>XNLAALRSELQALRREGFSPERLAALESRLQALERRLAALRSRLQALRGX[4x];>XGLCALRSELQALRREGFSPEELAALESELQALERELAALRSELQALRGX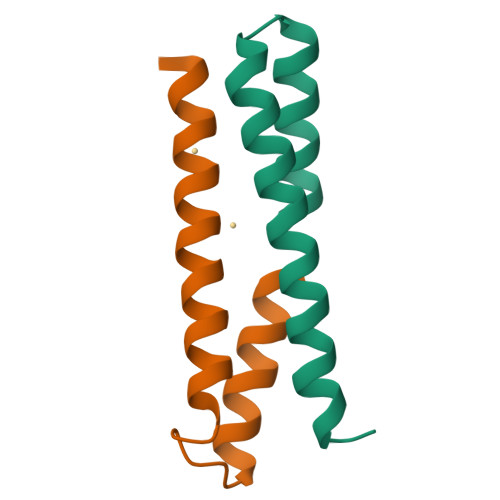[4x]>[4x]HHHHHHGTYFHSVNAGVIPPPALTDKLRLYHVDMNP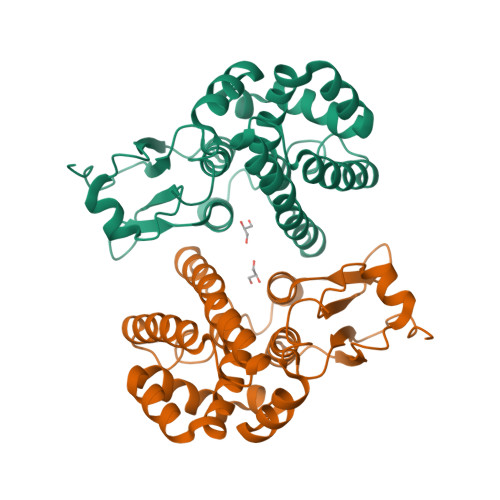YGHRVLLVLEAKRIKYEVYRLDPLRLPEWFRAKNPRLKIPVLEIPTDQGDRFLFESVVICDYLDEKYTRHTLHSHDPYVKAQDRLLIERFNELIKGSLECFDTNFAFGSEQIIQTLEIFEKELTNRGTNYFGGNRPGMLDYMVWPWVERLYLLRCVNDRKFVEKKSLFPNFADWGDQMQLDDIVKKHAHSPQEYFDYYKNARAHSMGYYL~{N}-methyl-~{N}-[3-[[[2-[(2-oxidanylidene-3,4-dihydro-1~{H}-quinolin-6-yl)amino]-5-(trifluoromethyl)pyrimidin-4-yl]amino]methyl]pyridin-2-yl]methanesulfonamide | C22 H22 F3 N7 O3 S | 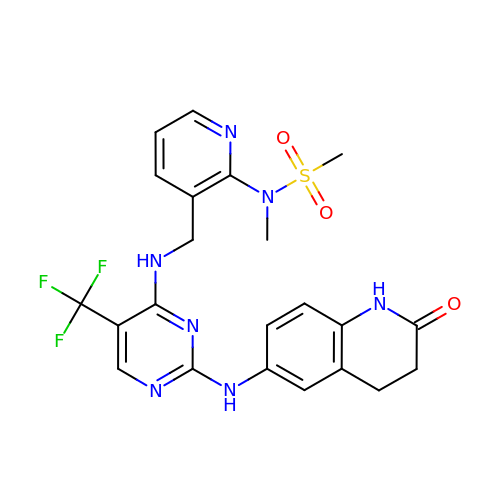MUVVMGFRHXQCRG-UHFFFAOYSA-N>[2x]TKGTIYLTFDDGPINASIDVINVLNQEEVKATFYFNAWHLDGIGDENEDRALEALKLALDSGHIVANHSYDHMVHNCVEEF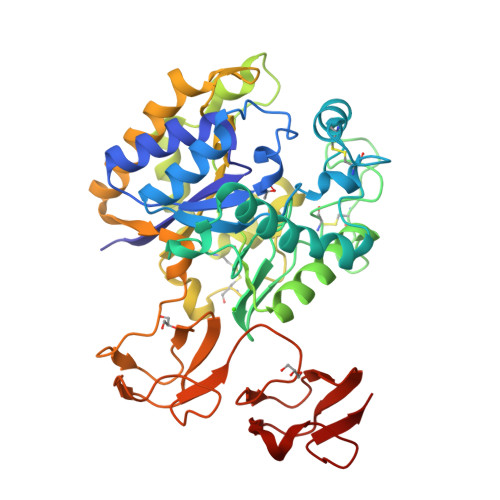GPNSAAECNATGDHQINSYQDPAYDASMFAENLSVLEKYLPNITSYPNYKANEFARLPYTNGWRVTKDFKADGLCATSDDLKPWEPGYACDTANPSNSVKAAIAVQNILANNGYQTHGWDVDWAPENWGIAMPANSLTEAEPFLGYVDSALNTCAPTTINPINSKAQEFPCGTPLHADKVIVLTHEFLFEDGKRGMGATQNLPKLTKFIQLAKQAGYVFDTMDNYTPNWQVGNNYSAGDYVLHLGTVYQAVTSHTAQQDWAPSPTSSLWTNADPATNWTQNVSYKQGDVVTYQGLRYLVNVPHVSQADWSPSSQNTLFTAL>[4x]AGGLSQLVAYGAQDVYLTGNPQITFFKTVYRRYTNFAIESIQQTINGSVGFGNK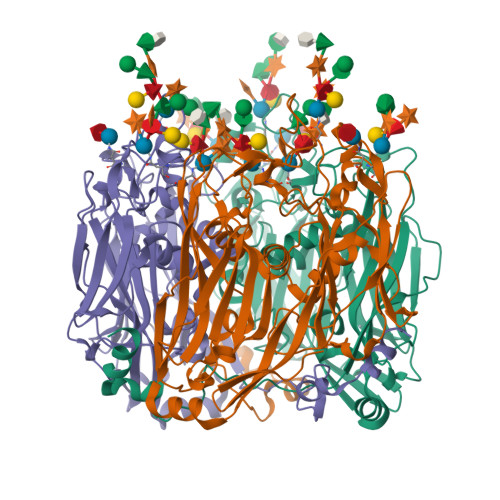VSTQISRNGDLITDIVVEFVLTKGGNGGTTYYPAEELLQDVELEIGGQRIDKHYNDWFRTYDALFRMNDDRYNYRRMTDWVNNELVGAQKRFYVPLIFFFNQTPGLALPLIALQYHEVKLYFTLASQVQGVNYNGSSAIAGAAQPTMSVWVDYIFLDTQERTRFAQLPHEYLIEQLQFTGSETATPSATTQASQNIRLNFNHPTKYLAWNFNNPTNYGQYTALANIPGACSGAGTAAATVTTPDYGNTGTYNEQLAVLDSAKIQLNGQDRFATRKGSYFNKVQPYQSIGGVTPAGVYLYSFALKPAGRQPSGTCNFSRIDNATLSLTYKTCSIDATSPAAVLGNTETVTANTATLLTALNIYAKNYNVLRIMSGMGGLAYAN> MPEDQVGKLEATENTISAMAAAAAEQQQFYLLLGNLLSPDNVVRKQAEETYENIPGQSKITFLLQAIRNTTAAEEARQMAAVLLRRLLSSAFDEVYPALPSDVQTAIKSELLMIIQMETQSSMRKKVCDIAAELARNLIDEDGNNQWPEGLKFLFDSVSSQNVGLREAALHIFWNFPGIFGNQQQHYLDVIKRMLVQCMQDQEHPSIRTLSARATAAFILANEHNVALFKHFADLLPGFLQAVNDSCYQNDDSVLKSLVEIADTVPKYLRPHLEATLQLSLKLCGDTSLNNMQR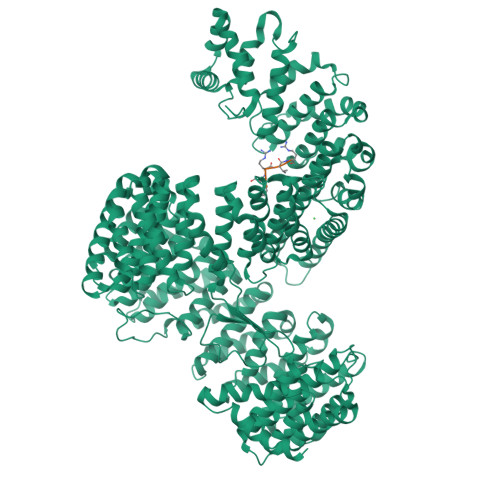QLALEVIVTLSETAAAMLRKHTNIVAQTIPQMLAMMVDLEEDEDWANADELEDDDFDSNAVAGESALDRMACGLGGKLVLPMIKEHIMQMLQNPDWKYRHAGLMALSAIGEGCHQQMEGILNEIVNFVLLFLQDPHPRVRYAACNAVGQMATDFAPGFQKKFHEKVIAALLQTMEDQGNQRVQAHAAAALINFTEDCPKSLLIPYLDNLVKHLHSIMVLKLQELIQKGTKLVLEQVVTSIASVADTAEEKFVPYYDLFMPSLKHIVENAVQKELRLLRGKTIECISLIGLAVGKEKFMQDASDVMQLLLKTQTDFNDMEDDDPQISYMISAWARMCKILGKEFQQYLPVVMGPLMKTASIKPEVALLDTQDMENMSDDDGWEFVNLGDQQSFGIKTAGLEEKSTACQMLVCYAKELKEGFVEYTEQVVKLMVPLLKFYFHDGVRVAAAESMPLLLECARVRGPEYLTQMWHFMCDALIKAIGTEPDSDVLSEIMHSFAKCIEVMGDGCLNNEHFEELGGILKAKLEEHFKNQELRQVKRQDEDYDEQVEESLQDEDDNDVYILTKVSDILHSIFSSYKEKVLPWFEQLLPLIVNLICPHRPWPDRQWGLCIFDDVIEHCSPASFKYAEYFLRPMLQYVCDNSPEVRQAAAYGLGVMAQYGGDNYRPFCTEALPLLVRVIQSADSKTKENVNATENCISAVGKIMKFKPDCVNVEEVLPHWLSWLPLHEDKEEAVQTFNYLCDLIESNHPIVLGPNNTNLPKIFSIIAEGEMHEAIKHEDPCAKRLANVVRQVQTSGGLWTECIAQLSPEQQAAIQELLNSA;> FRVR>[2x]AYTQQPGAPWGLGRISHRSKGSTTYEYDTSGGSGTCAYVIDTGVEASHPEFEGRASQIKSFISGQNTDGNGHGTHCAGTIGSKTYGVAKKTKIYGVKVLDNSGSGSYSGIISGMDFAVQDSKSRSCPKGVVANMSLGGGKAQSVNDGAAAMIRAGVFLAVAAGNDNANAANYSPASEPTVCTVGATTSSDARSSFSNYGNLVDIFAPGSNILSTWIGGTTNTISGTSMA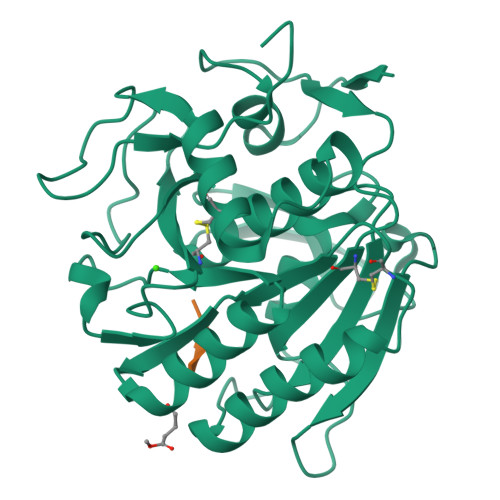TPHIVGLGAYLAGLEGFPGAQALCKRIQTLSTKNVLTGIPSGTVNYLAFNGNPSG;>[2x]XAAPV> HHHHASILIDTSAWVEYFRATGSIAAVEVRRLLSEEAARIAMCEPIAMEILSGALDDNTHTTLERLVNGLP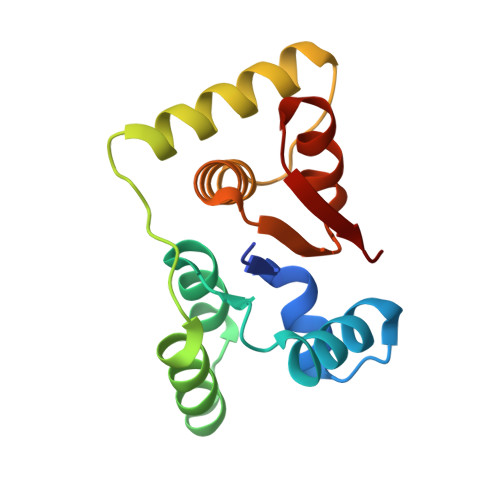SLNVDDAIDFRAAAGIYRAARRAGETVRSINDCLIAALAIRHGARIVHRDADFDVIARITNLQAASFR> QGFSLAQYLQEQKTIVETALDQSLVITEPVTIYEAMRYSLLAGGKRLRPILCLAACEMLGGTAAMAMNTACALEMIHTMSLIHDDLPAMDNDDLRRGKPTNHKVYGEDIAILAGDALLSYAFEYVARTPDVPAERLLQVIVRLGQAVGAEGLVGGQVVDLESEGKDVAVETLNFIHTHKTGALLEVCVTAGAILAGAKPEEVQLLSRYAQNIGLAFQIVDDILDITVTYPKSQAEAQKLVAEAIASLEPYGEKANPLKALAEYIVNA;> QGFSLAQYLQEQKTIVETALDQSLVITEPVTIYEAMRYSLLAGGKRLRPILCLAACEMLGGTAAMAMNTACALEMIHTMSLIHDDLPAMDNDDLRRGKPTNHKVYGEDIAILAGDALLSYAFEYVARTPDVPAERLLQVIVRLGQAVGAEGLVGGQVVDLESETDVAVETLNFIHTHKTGALLEVCVTAGAILAGAKPEEVQLLSRYAQNIGLAFQIVDDILSLEKSQAEAQKLVAEAIASLEPYGEKANPLKALAEYI;> QGFSLAQYLQEQKTIVETALDQSLVITEPVTIYEAMRYSLLAGGKRLRPILCLAACEMLGGTAAMAMNTACALEMIHTMSLIHDDLPAMDNDDLRRGKPTNHKVYGEDIAILAGDALLSYAFEYVARTPDVPAERLLQVIVRLGQAVGAEGLVGGQVVDLESEGVETLNFIHTHKTGALLEVCVTAGAILAGAKPEEVQLLSRYAQNIGLAFQIVDDILLWGIEKSQAEAQKLVAEAIASLEPYGEKANPLKALAEYI;> QGFSLAQYLQEQKTIVETALDQSLVITEPVTIYEAMRYSLLAGGKRLRPILCLAACEMLGGTAAMAMNTACALEMIHTMSLIHDDLPAMDNDDLRRGKPTNHKVYGEDIAILAGDALLSYAFEYVARTPDVPAERLLQVIVRLGQAVGAEGLVGGQVVDLESEGKTDVAVETLNFIHTHKTGALLEVCVTAGAILAGAKPEEVQLLSRYAQNIGLAFQIVDDILTYPSLWGIEKSQAEAQKLVAEAIASLEPYGEKANPLKALAEYI;> VADAHTQGFSLAQYLQEQKTIVETALDQSLVITEPVTIYEAMRYSLLAGGKRLRPILCLAACEMLGGTAAMAMNTACALEMIHTMSLIHDDLPAMDNDDLRRGKPTNHKVYGEDIAILAGDALLSYAFEYVARTPDVPA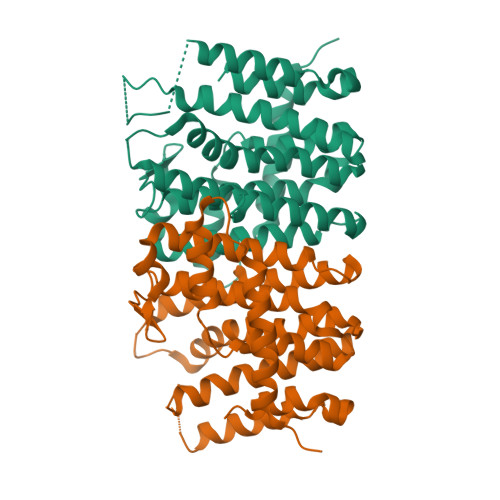ERLLQVIVRLGQAVGAEGLVGGQVVDLESEVAVETLNFIHTHKTGALLEVCVTAGAILAGAKPEEVQLLSRYAQNIGLAFQIVKSQAEAQKLVAEAIASLEPYGEKANPLKALAEYIVNR;> QGFSLAQYLQEQKTIVETALDQSLVITEPVTIYEAMRYSLLAGGKRLRPILCLAACEMLGGTAAMAMNTACALEMIHTMSLIHDDLPAMDNDDLRRGKPTNHKVYGEDIAILAGDALLSYAFEYVARTPDVPAERLLQVIVRLGQAVGAEGLVGGQVVDLESEGKETLNFIHTHKTGALLEVCVTAGAILAGAKPEEVQLLSRYAQNIGLAFQIVDDSQAEAQKLVAEAIASLEPYGEKANPLKALAEYIVNR>YANPVWTALFDYEPSGQDELALRKGDRVEVLSRDAAISGDEGWWAGQVGGQVGIFPSNYVSRGGGAPPIPPPR[2x]

MLK3, also known as MAP3K11, is a serine/threonine protein kinase involved in regulating the JNK, p38, and ERK pathways. It is composed of several modules: an SH3 domain, a kinase domain, tandem leucine zippers, a Cdc42/Rac interactive binding (CRIB) motif, several linker regions, and a proline-rich C-terminal tail. The SH3 domain has been implicated in the autoinhibition of the kinase domain through an intramolecular interaction via a nonconsensus single proline motif located between the leucine zipper and CRIB motif in the full-length MLK3 protein. The overall structure reveals a five-stranded antiparallel β-barrel, a characteristic of all known SH3 domains, and three loops (RT, n-Src, and 310 helix), commonly involved in the recognition of both proline-rich and nonproline ligands.

In this study, we also mapped the location of the canonical binding site on MLK3 SH3 by solving a structure of the SH3 domain of MLK3 bound to the NS5A-derived peptide (APPIPPPR). The crystals diffracted to 1.5 Å with an Rwork/Rfree of 18.8%/22.8%. The NS5A sequence crystallized here is from a different genotype of HCV but carries the same PXXPXR motif that is conserved across all HCV genotypes. The NS5A peptide interacts with the canonical polyproline-binding site by forming contacts with residues Asp-58 and Glu-59 of the RT loop, residues Asn-98 and Tyr-99 of the 310 helix, residues Asp-80 of the n-Src loop, and residue Trp-83 of the β3 strand from MLK3 SH3. Alignment of both complexes shows that the two binding sites are on the opposite faces of the SH3 domain. Interestingly, Asp-80 and Trp-83 of the MLK3 SH3 domain participate in binding both peptides; however, in the case of Trp-83, the side chain is implicated in interactions with the NS5A peptide, whereas its backbone carbonyl interacts with MIP. The Asp-80 side chain is the only one involved in both interactions; it is oriented differently depending on which peptide is bound and interacts with arginine residues present in both peptides. Finally, the shift in the n-Src loop required for MIP binding likely interferes with the binding of NS5A, further explaining the competition between the two peptides.> GLPTMNTPGSNQFLTSDDFQSPCALPNFDVTPPIHIPGEVKNMMELAEIDTLIPMNAVDGKVNTMEMYQIPLNDNLSKAPIFCLSLSPASDKRLSHTMLGEILNYYTHWTGSIRFTFLFCGSMMATGKLLLSYSPPGAKPPTNRKDAMLGTHIIWDLGLQSSCSMVAPWISNTVYRRCARDDFTEGGFITCFYQTRIVVPASTPTSMFMLGFVSACPDFS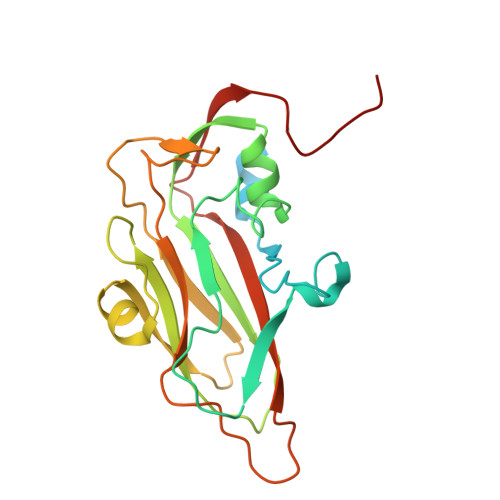VRLLKDTPHISQSK>[4x]MGSSHHHHHHSSGLVPRGSHSNYGKSADGTVTIEYFNQKKEMTKTLEEITRDFEKENPKIKVKVVNVPNAGEVLKTRVLAGDVPDVVNIYPQSIELQEWAKAGVFEDLSNK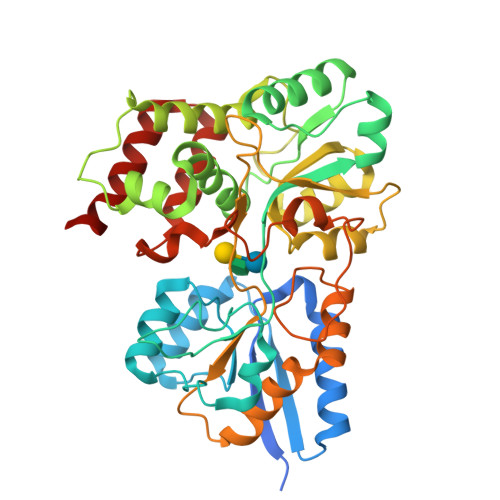DYLKRVKNGYAEKYAVNEKVYNVPFTANAYGIYYNKDKFEELGLKVPETWDEFEQLVKDIVAKGQTPFGIAGADAWTLNGYNQLAFATATGGGKEANQYLRYSQPNAIKLSDPIMKDDIKVMDILRINGSKQKNWEGAGYTDVIGAFARGDVLMTPNGSWAITAINEQKPNFKIGTFMIPGKEKGQSLTVGAGDLAWSISATTKHPKEANAFVEYMTRPEVMQKYYDVDGSPTAIEGVKQAGEDSPLAGMTEYAFTDRHLVWLQQYWTSEADFHTLTMNYVLTGDKQGMVNDLNAFFNPMKADVD Protein stability can be fine‐tuned by modifying different structural features such as hydrogen‐bond networks, salt bridges, hydrophobic cores, or disulfide bridges. Among these, stabilization by salt bridges is a major challenge in protein design and engineering since their stabilizing effects show a high dependence on the structural environment in the protein, and therefore are difficult to predict and model. In this work, we explore the effects on structure and stability of an introduced salt bridge cluster in the context of three different de novo TIM barrels. The results show that despite the similarities in protein fold, the salt bridge clusters differently influence the structural and stability properties of the de novo TIM barrel variants depending on the structural background where they are introduced.

The salt bridge variants exhibit similar thermostability in comparison with their parental designs but important differences in the conformational stability at 25°C can be observed such as a highly stabilizing effect for two of the proteins but a destabilizing effect to the third. Analysis of the formed geometries of the salt bridge cluster in the crystal structures show either highly ordered salt bridge clusters or only single salt bridges. Rosetta modeling of the salt bridge clusters results in a good prediction of the tendency on stability changes but not the geometries observed in the three‐dimensional structures.

> MDVDEMLKQVEILRRLGAKRIAVRSDDWRILQEALKKGGDILIVDATDVDEMLKQVEILRRLGAKEIAVRSDDWRILQEALKKGGDILIVDATDVDEMLKQVEILRRLGAKRIAVRSDDWRILQEALKKGGDILIVDATDVDEMLKQVEILRRLGAKEIAVRSDDWRILQEALKKGGDILIVDATLEHHHHHH>[2x]GQEIRPMPADSAYGVVHISVCNMRDEGKFTSGMSTQALLGMPVKVLQYTGWYEIQTPDDYTGWVHRMVITPMSKEKYDEWNRAEKIVVTSHYGFTYEKPDDDSQTVS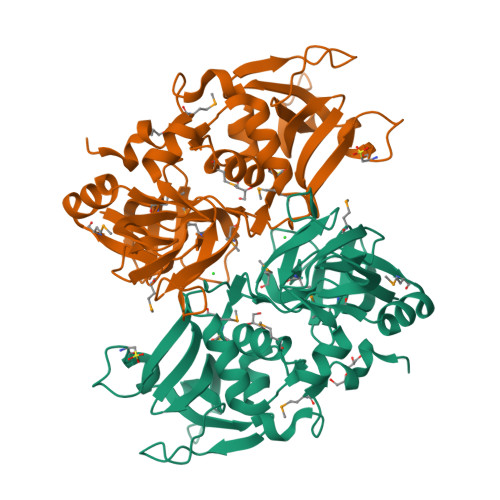DVVAGNRLKWEGSKGHFYKVSYPDGRQAYISRHISQPESKWRASLKQDAESIIKTAYTMIGIPYLWAGTSSKGVDCSGLVRTVLFMHDIIIPRDASQQAYVGERIEIAPDFSNVQRGDLVFFGRKATADRKEGISHVGIYLGNKRFIHALGDVHISSFDPEDECYDEFNTGRLLFATRFLPYINKEKGMNTTDHNLYYLHH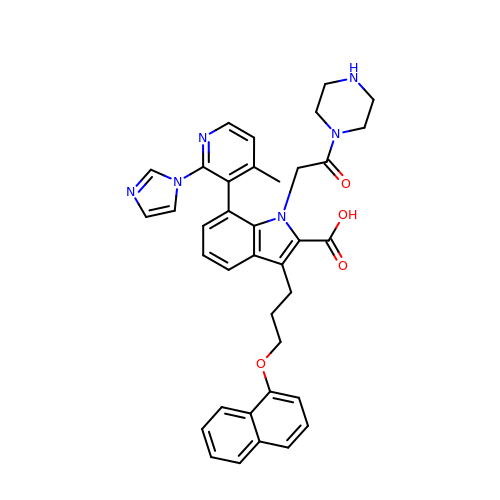7-[2-(1H-imidazol-1-yl)-4-methylpyridin-3-yl]-3-[3-(naphthalen-1-yloxy)propyl]-1-[2-oxo-2-(piperazin-1-yl)ethyl]-1H-indole-2-carboxylic acid | C37 H36 N6 O4 | ZZKICOFWGKKSRR-UHFFFAOYSA-N>[4x]GDSIEDKNARVIELIAAYRNRGHLMADIDPLRLDNTRFRSHPDLDVNSHGLTLWDLDREFKVDGFAGVQRKKLRDILSVLRDAYCRHVGVEYTHILEPEQQRWIQERVETKHDKPTVAEQKYILSKLNAAEAFETFLQTKYVGQKRFSLEGAETVIPMMDAVIDQCAEHGLDEVVIAMPHRGRLNVLANIVGKPYSQIFSEFEGNLNPSQAHGSGDVKYHLGATGTY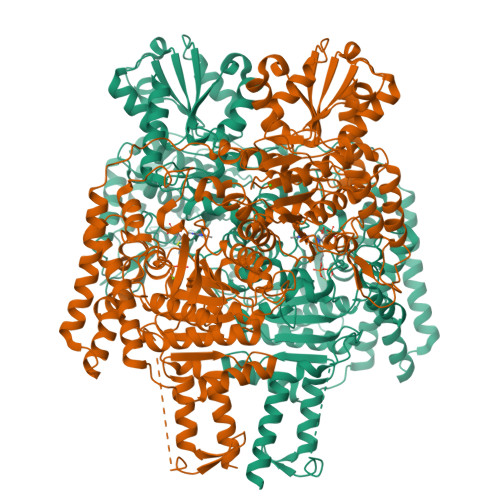IQMFGDNDIEVSLTANPSHLEAVDPVLEGLVRAKQDLLDTGEEGSDNRFSVVPLMLHGDAAFAGQGVVAETLNLALLRGYRTGGTIHIVVNNQIGFTTAPTDSRSSEYCTDVAKMIGAPIFHVNGDDPEACAWVARLAVDFRQAFKKDVVIDMLCYRRRGHNEGDDPSMTQPYMYDVIDTKRGSRKAYTEALIGRGDISMKEAEDALRDYQGQLERVFNEVRELEKHEIEPSESVEADQQIPSKLATAVDKAMLQRIGDAHLALPEGFTVHPRVRPVLEKRREMAYEGRIDWAFAELLALGSLIAEGKLVRLSGQDTQRGTFTQRHAVIVDRKTGEEFTPLQLLATNPDGTPTGGKFLVYNSALSEFAAVGFEYGYSVGNPDAMVLWEAQFGDFVNGAQSIIDEFISSGEAKWGQLSDVVLLLPHGHEGQGPDHTSGRIERFLQLWAEGSMTIAMPSTPANYFHLLRRHGKDGIQRPLIVFTPKSMLRNKAAVSDIRDFTESKFRSVLEEPMYTDGEGDRNKVTRLLLTSGKIYYELAARKAKENREDVAIVRIEQLAPLPRRRLAETLDRYPNVKEKFWVQEEPANQGAWPSFGLTLPEILPDHFTGLKRISRRAMSAPSSGSSKVHAVEQQEILDTAFG>SSVDDMYDFICSGPLISKIGLTPEKVAESIDEWIEYGLRLCRLFQLNQLSLNEAQKIRIYHYYIPVFMWCEQEISQHSSKFKEEEEIPPLVIGFSAPQGCGKTTLVFALEYLFKITGRKAATMSIDDFYLTAEEQAKLRDSNPGNLLLEFRGNAGSHDLPFSVETMTALSKLTKEGVKVKLPRYDKSAYSGRGDRADPSEWPEVEGPLPVILFEGWMLGFKPLPPEVVKAVDPQLETINKNMEAYYDAWHKYVKSWIVIKIQDPSYVYQWRLQAEIAMRADGKPGMSDEEVKDFVS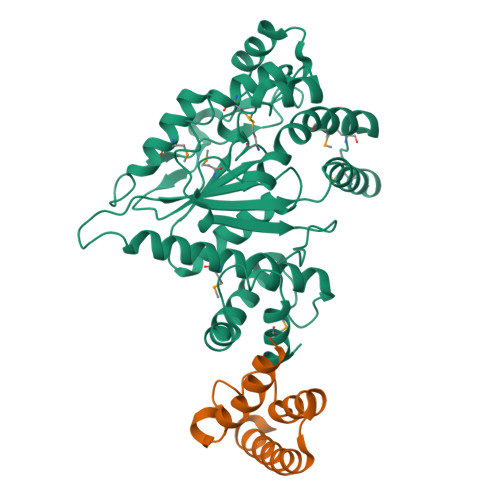RYMPAYKAYLPTLYSEGPSGSDPKHVLLIDIDEGRNPILGC[2x];>STQNLGNSLMRVFSKEATRKYYLDLFKRADFTANLPKLAKKGGPDRLNDALKKLRKAGISEEKFAELKGAAAKYADDWYRIYGK[2x]>[2x]MNDLERLFNPSAIAVVGASKDPSKIGSQILRNLLSYGFKGKVYPINPTADELMGLKCYPKVSDVPDKVDVAVISVPSDKVLGVIDDCGKAGVKFAVVITSGFKEVGNEELEEELVRRAHSYGMRVLGPNIFGYLYAPARLNATFGPKDVLSGNVAFISQSGALGIALMGYTVVENIGISSIVSVGNKADLDDVDLLDFFDKDPNTGVIMIYLEGIAPGRGRMFIDVASRVSLRKPIIVIKAGRTEVGARAAASHTGSIAGSVAIYESAFKQSGILMAKSVEDAFDWTKALSWNPIPEGERLIVLTNGGGAGVQSTDTFADNGIYLSKPPESLIQEIKKFVPPFASFANPIDITGMAPDDWYYMGTLAALKNPDVDALTVLYCQTAVTTPIGVAKGIVDAIKEAGNSKPVTVGMVGGPEVAEAVSFLNKQRIAAYPTPERASSAMSALYAYARARSYVMKSLAVR;>MSSRDLLLKAKENGRKSLLEHEAKYFIS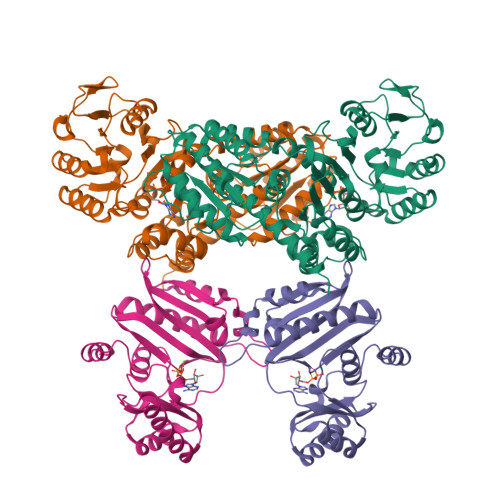SYGIPVTNIRLAKSEEEAVNFSREIGFPVVLKIVSPQVVHKSDVGGVKVNLRSEEEVRKAYREIIENVKRNVPNAEIEGILVQEFAPPGVELIIGLLRDPQFGPTVMFGLGGVFVELFRDVSFRVAPLSEQDAESMIKEVKAYKLLTGFRGMEPVDIEAIKDALIRAGRIGVENEEIAEMDLNPVIAYPKGIKVVDARIILR[2x]>[2x]SLFELGKMILQ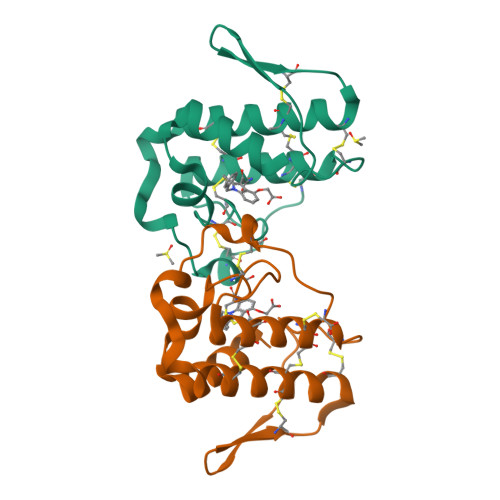ETGKNPAKSYGVYGCNCGVGGRGKPKDATDRCCYVHKCCYKKLTGCDPKKDRYSYSWKDKTIVCGENNSCLKELCECDKAVAICLRENLDTYNKKYRYNYLKPFCKKADPC>TPEMPVLENRAAQGNITAPGGARRLTGDQTAALRNSLSDKPAKNIILLIGDGMGDSEITAARNYAEGAGGFFKGIDALPLTGQYTHYALNKKTGKPDYVTDSAASATAWSTGVKTYNGALGVDIHEKDHPTILEMAKAAGLATGNVSTAELQHATPAALVAHVTSRKCYGPSATSQKCPGNALEKGGKGSITEQLLNARADVTLGGGAKTFAETATAGEWQGKTLREEAEARGYQLVSDAASLNSVTEANQQKPLLGLFADGNMPVRWLGPKATYHGNIDKPAVTCTPNPQRNDSVPTLAQMTDKAIELLSKNEKGFFLQVEGASIDK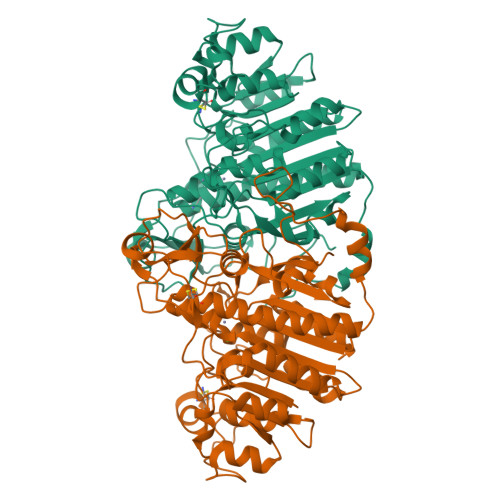QNHAANPCGQIGETVDLDEAVQRALEFAKKEGNTLVIVTADHAHASQIVAPDTKAPGLTQALNTKDGAVMVMSYGNSEEDSQEHTGSQLRIAAYGPHAANVVGLTDQTDLFYTMKAALGLK[2x]>MKDLVDTTEMYLRTIYELEEEGVTPLRARIAERLEQSGPTVSQTVARMERDGLVVVASDRSLQMTPTGRTLATAVMRKHRLAERLLTDIIGLDINKV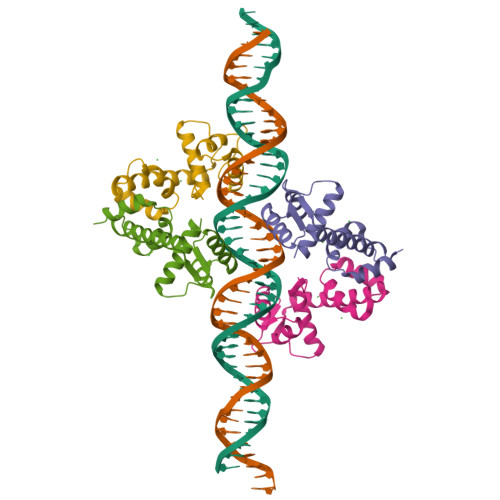HDEADRWEHVMSDEVERRLVKVLK[4x]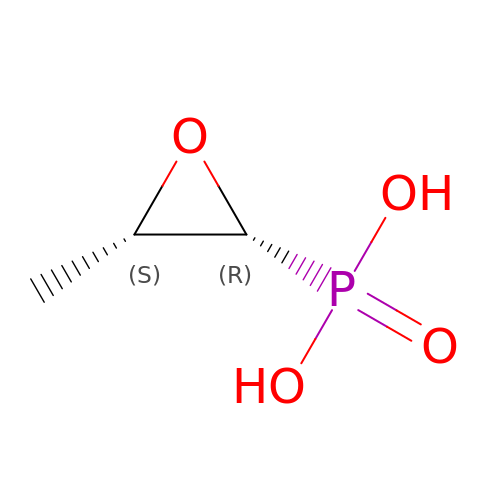FOSFOMYCIN | C3 H7 O4 P | YMDXZJFXQJVXBF-STHAYSLISA-N(3R,5R)-7-{3-(4-fluorophenyl)-1-(1-methylethyl)-4-phenyl-5-[(4-sulfamoylphenyl)carbamoyl]-1H-pyrrol-2-yl}-3,5-dihydroxyheptanoic 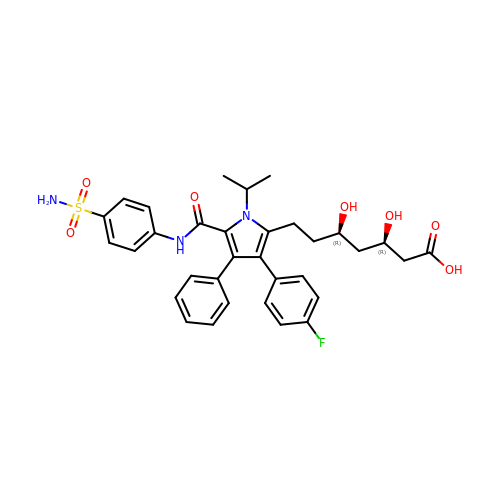acid | C33 H36 F N3 O7 S | ZBCQTJGKEZGMGJ-CLJLJLNGSA-N> MTIDQKNTNIDPRFPHHHPRPQSFWEARAKALESLLIEKGHLSSDAIERVIKHYEHELGPMNGAKVVAKAWTDPAFKQRLLEDSETVLRELGYYGLQGEHIRVVENTDT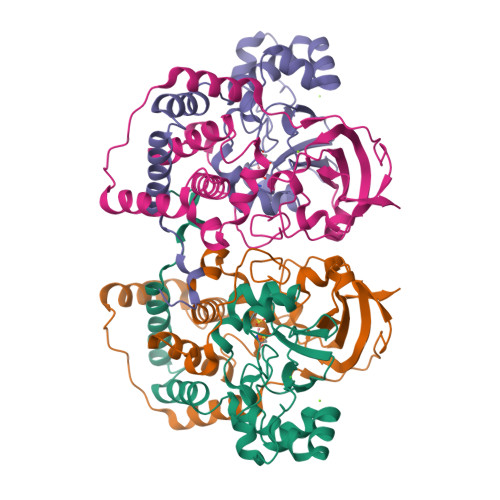VHNVVVCTLCSCYPWPLLGLPPSWYKEPAYRARVVKEPRQVLKEFGLDLPDSVEIRVWDSSSEIRFMVLPQRPEGTEGVTEEELAKLVTRDSMIGVAKIEPPKVTVG;> MNGIHDVGGMDGFGKVMYVKEEEDIYFTHDWERLAFGLVAGCMAQGLGMKAFDEFRIGIELMRPVDYLTSSYYGHWIATVAYNLVDTGVLDEKELEERTEVFLKKPDTKIPRREDPALVKLVEKALYDGLSPLREISASPRFKVGERIKTKNIHPTGHTRFPRYARVKYGVIDEVYGAHVFPDDAAHRKGENPQYLYRVRFEAEELWGYKQKDSVYIDLWESYMEPVSH>MESPRIELRSDITVELVDSSASDLAVVKAARVSTAGEDANDELYDGGSTRGLIRYLMRSRHGSPFEHNSMTFLVRAPIFTVRHLMRHRTWSFNEESARYREVGAAFYVPDATRLLRQEGKPGDYRYVGGSTDDHQQVVRSATR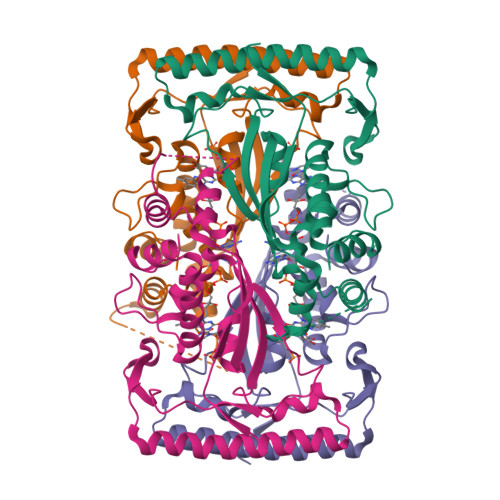AYEVAFEEYQRLLDSGIAREIARLVLPVSTYSVLYATCNARALMHFLSLRTHRPDAAYVSHPQREIEMVAEQMETAWAKLMPVTHEAFTAFGRVSP[4x]> GPLEDQEENTLRELRLFLRDVTKRLATDKRFNIFS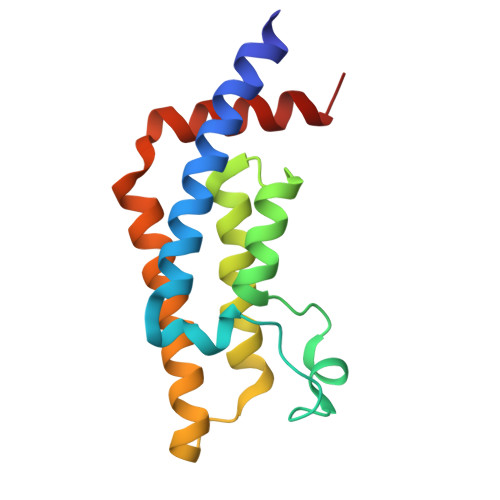KPVDIEEVSDYLEVIKEPMDLSTVITKIDKHNYLTAKDFLKDIDLICSNALEYNPDKDPGDKIIRHRACTLKDTAHAIIAAELDPEFNKLCEEIKEARIKR> GSGRGLGPLQIWQTDFTLEPRMAPRSWLAVTVDTASSAIVVT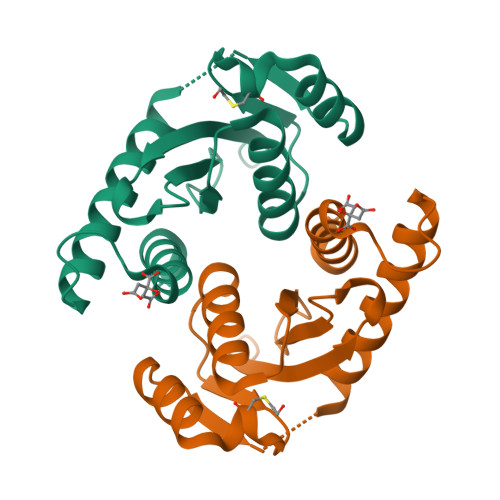QHGRVTSVAAQHHWATAIAVLGRPKAIKTDNGSCFTSKSTREWLARWGIAHTTGIPGNSQGQAMVERANRLLKDKIRVLAEGDGFMKRIPTSKQGELLAKAMYALNHF The Saccharomyces cerevisiae B-family replicative DNA polymerases, namely Pol ϵ, Pol δ and Pol α, have been estimated to incorporate about 13 000 NTPs during each cell cycle of the yeast genome, and Pol ϵ seems to incorporate the majority of NTPs, roughly four times as many ribonucleotides as Pol δ. Other examples where an amino acid adjacent to the steric gate residue influences ribonucleotide discrimination are found among B-family polymerases. It was first shown in the ϕ29 DNA polymerase that B-family polymerases have a conserved tyrosine (Y645 in Pol ϵ) that functions as a steric gate. Our data show that Pol ϵ discriminates NTPs through the concerted action of a steric gate residue (Y645) and a sensor in the finger domain (N828). A comparison with other B-family DNA polymerases showed that both Y645 and N828 are structurally conserved residues, thus reinforcing their functional importance.

To test the hypothesis that steric hindrance does not allow the finger domain to adopt a completely closed conformation when a ribonucleotide is bound to the active site, we replaced N828 with a valine, which is both less bulky and unable to form a hydrogen bond with the β-phosphate of the incoming nucleotide. The N828VPol2CORE-UTP structure showed a ribonucleotide bound to the active site in the presence of the steric gate, Y645 and showed that M644 provides stability to the active site in wild-type Pol ϵ. Compared to both the wild-type Pol2CORE-dATP and N828VPol2CORE-dATP structures, the presence of a ribonucleotide in the N828VPol2CORE structure did not induce any significant structural changes to the residues surrounding the ribonucleotide. The 2′-OH group of the sugar was lifted slightly upwards and away from the Y645 plane, but without affecting the finger domain as V828 remained unchanged in its position. A comparison between N828VPol2CORE-UTP and M644GPol2CORE-UTP showed that the less bulky V828 could accept a ribonucleotide in the active site without introducing any strain in the finger domain or tilting of the base in the ribonucleotide. In contrast, N828 shifted position and introduced a strain in the finger helix that might promote the opening of the finger domain followed by the dissociation of the ribonucleotide before a new bond is formed in the chemical step. When replacing N828 with a valine, a ribonucleotide is accepted by the active site. Despite an upward shift in the position of the sugar moiety, there is no clash between the V828 and the 2′-C of the ribose that would induce a strain in the finger domain. Thus, the finger domain is likely to be maintained in a closed state increasing the probability that chemistry will occur with a ribonucleotide in the active site.

>[2x]GGDPHMMFGKKKNNGGSSTARYSAGNKYNTLSNNYALSAQQLLNASKIDDIDSMMGFERYVPPQYNGRFDAKDIDQIPGRVGWLTNMHATLVSQETLSSGSNGGGNSNDGERVTTNQGISGVDFYFLDEEGGSFKSTVVYDPYFFIACNDESRVNDVEELVKKYLESCLKSLQIIRKEDLTMDNHLLGLQKTLIKLSFVNSNQLFEARKLLRPILQDNANNNVQRNIYNVAANGSEKVDAKHLIEDIREYDVPYHVRVSIDKDIRVGKWYKVTQQGFIEDTRKIAFADPVVMAFAIATTKPPLKFPDSAVDQIMMISYMIDGEGFLITNREIISEDIEDFEYTPKPEYPGFFTIFNENDEVALLQRFFEHIRDVRPTVISTFNGDFFDWPFIHNRSKIHGLDMFDEIGFAPDAEGEYKSSYCSHMDCFRWVKRDSYLPQGSQGLKAVTQSKLGYNPIELDPELMTPYAFEKPQHLSEYSVSDAVATYYLYMKYVHPFIFSLCTIIPLNPDETLRKGTGTLCEMLLMVQAYQHNILLPNKHTDPIERFYDGHLLESETYVGGHVESLEAGVFRSDLKNEFKIDPSAIDELLQELPEALKFSVEVENKSSVDKVTNFEEIKNQITQKLLELKENNIRNELPLIYHVDVASMYPNIMTTNRLQPDSIKAERDCASCDFNRPGKTCARKLKWAWRGEFFPSKMDEYNMIKRALQNETFPNKNKFSKKKVLTFDELSYADQVIHIKKRLTEYSRKVYHRVKVSEIVEREAIVCQRENPFYVDTVKSFRDRRYEFKGLAKTWKGNLSKIDPSDKHARDEAKKMIVLYDSLQLAHKVILVSFYGYVMRKGSRWYSMEMAGITCLTGATIIQMARALVERVGRPLELDTDGIWCILPKSFPETYFFTLENGKKLYLSYPCSMLNYRVHQKFTNHQYQELKDPLNYIYETHSENTIFFEVDGPYKAMILPSSKEEGKGIKKRYAVFNEDGSLAELKGFELKRRGELQLIKNFQSDIFKVFLEGDTLEGCYSAVASVCNRWLDVLDSHGLMLEDEDLVSLICENRSMSKTLKEYEGQKSTSITTARRLGDFLGEDMVKDKGLQCKYIISSKPFNAPVTERAIPVAIFSADIPIKRSFLRRWTLDPSLEDLDIRTIIDWGYYRERLGSAIQKIITIPAALQGVSNPVPRVEHPDWLKRKIAT> SMKPTKVHIGRLTRNVTKDHIMEIFSTYGKIKMIDMPVERMHPHLSKGYAYVEFENPDEAEKALKHMDGGQIDGQEITATAVLAPW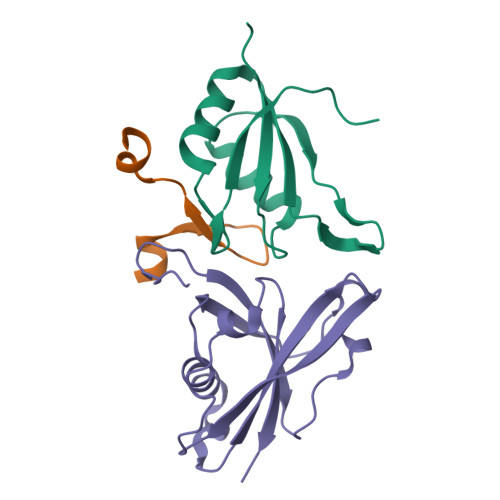PR;> KENEPPIRLLDDLFRKTKGTPCIYWLPLTPEAIAEKEAFR;> KEPEKPIDREKTCPLLLRVFTTNNGRHHRMDEFSRGNVPSSELQIYTWMDATLKELTSLVKEVYPEARKKGTHFNFAIVFMDLKRPGYRVKEIGSTMSGRKGTDDSMTLQSQKFQIGDYLDIAITPPNRA>[2x]GMNESSTHDSVADDPTEVSTDTVLDIALSLFSELGFSDAKLEAIAKKSGMSKRMIHYHFGDKRGL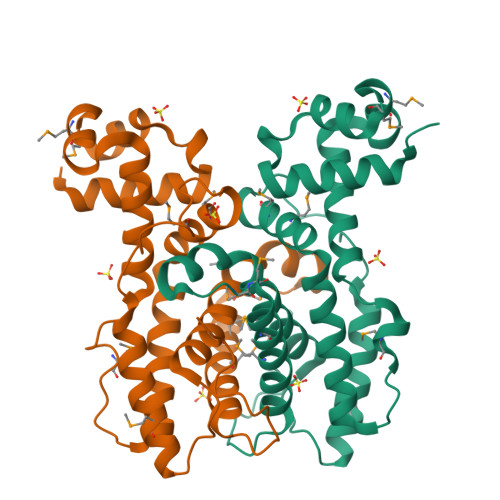YICCLEEAVRRLRPTAEEMYLASAVPVEGVRTIVEAVFHRYVQHPEAVRMLQMENLHHYGKVAEASPLSDQSAITLQLDRLLMLGQDAGAFRPGISAQDVFTLIASIAVFRINSRSTTLNLYGIDMMNGDNTDGMRRMAVDTVLAFLTSNLKSADEDSYLSRPLLSTVTEHVDEEGSYEVAADPFS>MANKGRLGEQEAFAMTVPLLIDVDSSQQEALEAIALNDELVRVRRALYLDLGVPFPGIHLRFNEGMGEGEYLISLQEVPVARGELKAGYLLVRESVSQLELLGIPYEKGEHLLPDQ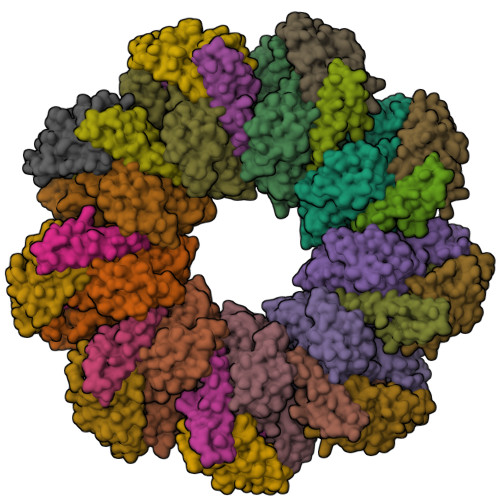ETFWVSVEYEERLEKSQLEFFSHSQVLTWHLSHVLREYAEDFIGIQETRYLLEQMEGGYGELIKEVQRIVPLQRMTEILQRLVGEDISIRNMRSILEAMVEWGQKEKDVVQLTEYIRSSLKRYICYKYANGNNILPAYLFDQEVEEKIRSRVRQTSAGSYLALDPAVTESLLEQVRKTIGDLSQIQSKPVLIVSMDIRRYVRKLIESEYYGLPVLSYQELTQQINIQPLGRVCL[18x];>[18x]GAMGALPPDGHPVEPHLERLYPTAQSKRSLWDFASPGYTFHGLHRAQDYRRELDTLQSLLTTSQSSELQAAAALLKCQQDDDRLLQIILNLLHKV;>MGHHHHHHGNITLTKRQQEFLLLNGWLQLQCGHAERACILLDALLTLNPEHLAGRRCRLVALLNNNQGERAEKEAQWLISHDPLQAGNWLCLSRAQQLNGDLDKARHAYQHYLELKDHNESP[18x]> GSPEFMIGEEVPSDQYYWAPLAQHERGSLASLDSLRKGGPPPPNWRQPELPEVIAMLGFRLDAVKSNAAAYLQHLCYRNDKVKTDVRKLKGIPVLVGLLDHPKKEVHLGACGALKNISFGRDQDNKIAIKNCDGVPALVRLLRKARDMDLTEVITGTLWNLSSHDSIKMEIVDHALHALTDEVIIPHSGWEREPNEDCKPRHIEWESVLTNTAGCLRNVSSERSEARRKLRECDGLVDALIFIVQAEIGQKDSDSKLVENCVCLLRNLSYQVHREIPQAERYQEAAPNVANNTGTSPARGYELLFQPEVVRIYISLLKESKTPAILEASAGAIQNLCAGRWTYGRYIRSALRQEKALSAIADLLTNEHERVVKAASGALRNLAVDARNKELIGKHAIPNLVKNLPGGQQNSSWNFSEDTVISILNTINEVIAENLEAAKKLRETQGIEKLVLINKSGNRSEKEVRAAALVLQTIWGYKELRKPLEKEGWKKSDFQVNLNNASRSQSSHSYDDSTLPLIDRNQKSDKKPDREEIQMS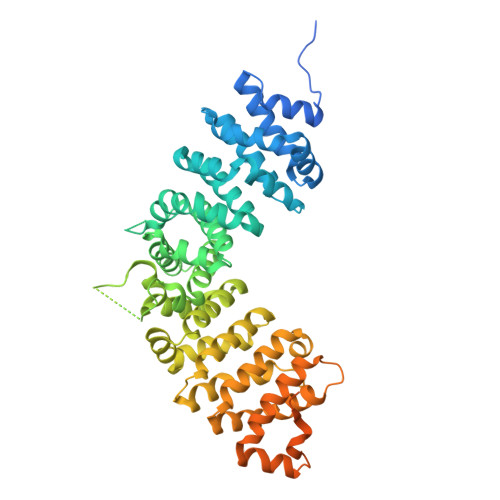NMGSNTKSLDNNYSTPNERGDHNRTLDRSGDLGDMEPLKGTTPLMQKI> MAENDFGIAIIGMAGRFPQADTVQAFWENLLASRECISFYSDEELLAMGISPEFVQHPDYVKAKGEVADIDKFDAAFFGIAPREAELMDPQHRVLLETAWAAFEDAGYVAADYPGDVGIFAGKSMDSYLMLNLMPHFKRVFSSGSLQAAIGNDKDSITTTIAYHLNLRGPAITVQTSSSTSLVAVCVACQSLLTWQCDMAIAGGVTLGPPAKTGYLSQEGGITAADGHCRAFSDNSSGFVPGTGAGLVVLKRVDEALRDGDNIYAVIKGFAVNNDGSEKISYTAPSVDAQARAIAQAQRLAGLTPQDITYVEAHGTGTRLGDPVEFSALSQAFAGASQKQYCALGSVKTNIGHLDTAAGVAGLIKTALAVQQGIIPATLHFERPNAQIDLTNSPFYINTTCQPWQPESGIRRAGVTSLGMGGTNAHVVLEQAPAVDLQARAPVPAYSILPFSAKTDSALSSGLARFADFLQHESLPDRRDLAWTLSQGRKAFAHRAALVTRDLHAAGTLLQQAATAPFARGVAQTQLGLGLLFSGQGSQYQRMGHQLYQVWPAYADAFDRCATLLEREYQLDIRHELFRAEVSLAQGERLAQTCLTQPLLFSVEYALAQLWLSWGITPTVMIGHSLGEWVAATLAGVFSLEDALRLVARRAELMHQAPSGAMLMVALPEAQIRALITAPLAIAAVNAPDYSVIAGPTSEILAVSQRLTEQNIINKRLHTSHAFHSSMMQDAAQALRQAFENVRLNPPTLTIISTVTGAHVSADTLTTPDYWIEQMLMPVQFSAALQEAQATFDVDFLEIGPGATLTQLTNGHALGDRLAFSSLPAGARS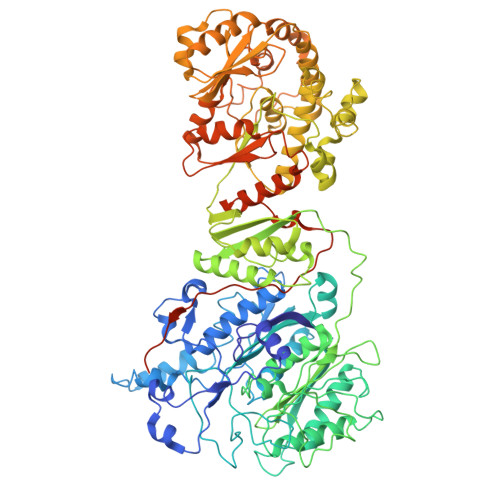SDEHKHILDTVAALWVRGHNIDLSAFAGEQPRRVSLPTYAFDKIRYWVDSPEEQRSAVTPVADAGSKLSSGLEVLFQGPSSGHHHHHHHHHH>MEDGKRLRIGITLHPYYSYVSNIVGDKAEVVPLIPAGFNPHAYEPRAEDIKRIGTLDVVVLNGVGHDDFAERMIASSEKPGIPVIEANAKVPLLAATGMAARGAGKVVNPHTFLSISASITQVNTIARELGKLDPANAKAYTRNARAYAKRLRALRADALARLNKA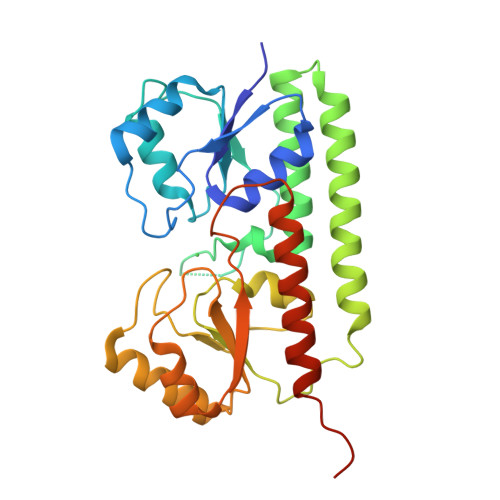PAADFRVATIHGAYDYLLREFGLEVTAVVEPAHGIEPSPSQLKKTIDQLKALDVKVIFSEIDFPSTYVETIQRESGVKLYSLSHISYGDYSAGKYEEEMARNLDTVVRAIQESGAEILYFQSHHHHHH[2x]3,7-DIHYDROXY-2-NAPHTHOIC ACID | C11 H8 O4 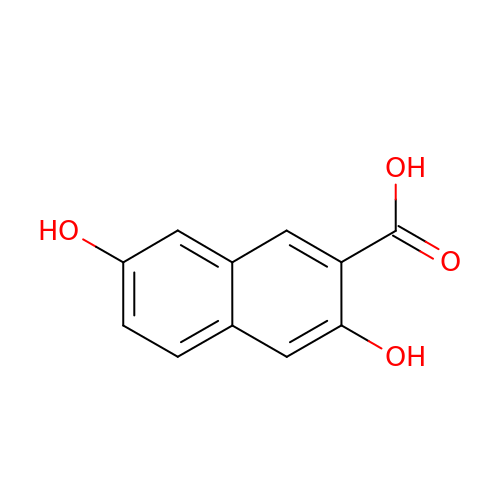| QMWOUSYSNFCKAZ-UHFFFAOYSA-N>[6x]MKIALTNLPPEHGE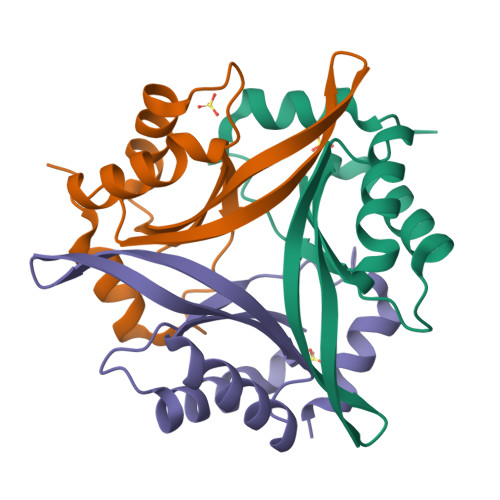RIARLLVEEHIVACVNLYPVHSIYSWKGEVCSEAEVTLMMKVSTQGIERLKQRICELHPYELPEFVVIEVDNNASLREYIDFVKGETHLYSAWSHPQFEK>MKQYQMYVGGEWIDASNGQTEPVVSPINEEVLAYIQDADASDAERVLAVATTAQKEWAKQPARQRAEVLRKFAQLIRDNKQYLAELLVKEQGKLLKVALGEVEATSTFIEYACDWARQMDGDIVKSDNANEQIMIHKIPRGVVVAITAWNFPLALAGRKIGPALVAGNSIVVKPTSETPLATLELGYLAEQAGIPAGVLNIVTGGGRTLGNELVGHRMTNMVSMTGSTPAGQSIIRASANNMAHVQLELGGKAPFIVMEDADLEQAAAAALHSRFDNCGQVCTCNERMYVHGAVYDEFMRIFMGKVEAIKVGDPMDPASDMGPKVNANELAHMEELVAEAVDEGATVLFGGKKLEGPEFEKGFWFEPTVLTNVTQDMTIVHEESFGPILPVIKFDSFDEVIEYANDSDYGLAAMICTQNMHYINRLLTELESGEIYVNRGHGEQHQGFHNGYKLSGTGGEDGKYGFEQYLEKKTFYIN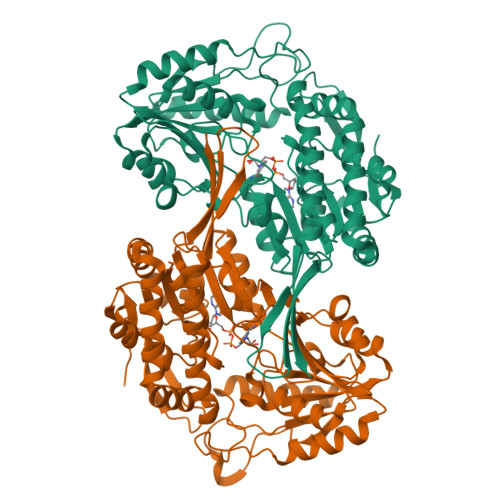YNLEHHHHHH[2x]> UGC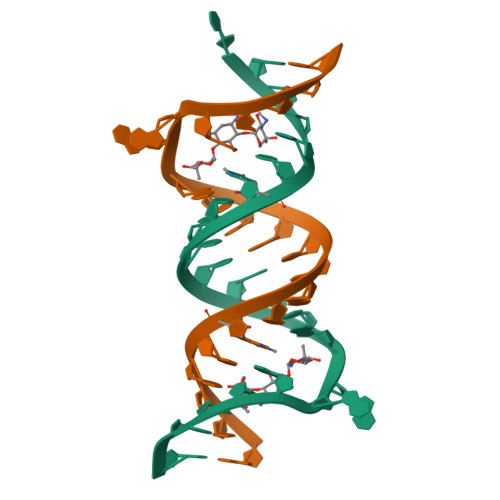GUCACGUCGACGAAGUCGC;> GCGUCACGUCGACGAAGUCGC> MVGSLNCIVAVSQNMGIGKNGDLPWPPLRNEFRYFQRMTTTSSVEGKQNLVIMGKKTWFSIPEKNRPLKGRINLVLSRE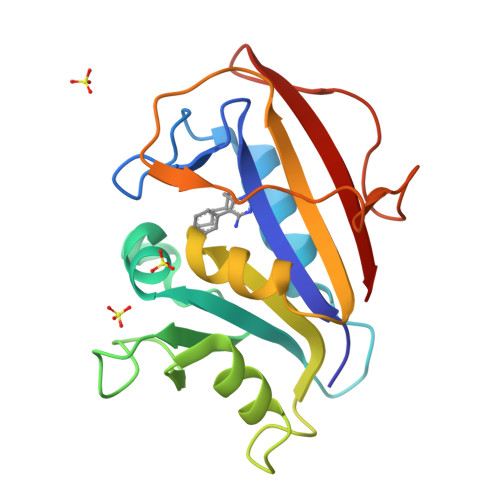LKEPPQGAHFLSRSLDDALKLTEQPELANKVDMVWIVGGSSVYKEAMNHPGHLKLFVTRIMQDFESDTFFPEIDLEKYKLLPEYPGVLSDVQEEKGIKYKFEVYEKND> GSKNIVNTSILSIVYKKDDLI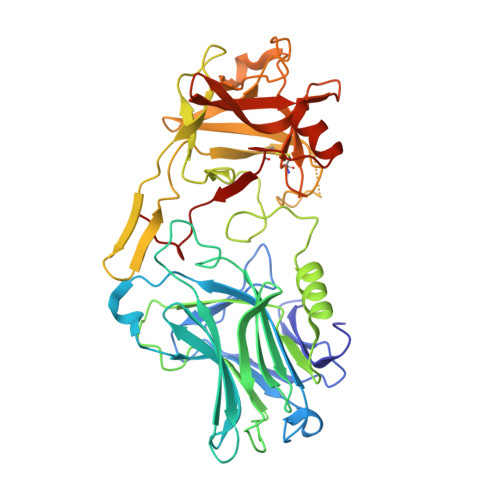DLSRYGAKINIGDRVYYDSIDKNQIKLINLESSTIEVILKNAIVYNSMYENFSTSFWIKIPKYFSKINLNNEYTIINCIENNSGWKVSLNYGEIIWTLQDNKQNIQRVVFKYSQMVNISDYINRWIFVTITNNRLTKSKIYINGRLIDQKPISNLGNIHASNKIMFKLDGCRDPRRYIMIKYFNLFDKELNEKEIKDLYDSQSNSGILKDFWGNYLQYDKPYYMLNLFDPNKYVDVNNIGIRGYMYLKGPRGSVVTTNIYLNSTLYEGTKFIIKKYASGNEDNIVRNNDRVYINVVVKNKEYRLATNASQAGVEKILSALEIPDVGNLSQVVVMKSKDDQGIRNKCKMNLQDNNGNDIGFIGFHLYDNIAKLVASNWYNRQVGKASRTFGCSWEFIPVDDGWGESSL2-oxopentanoic acid | C5 H8 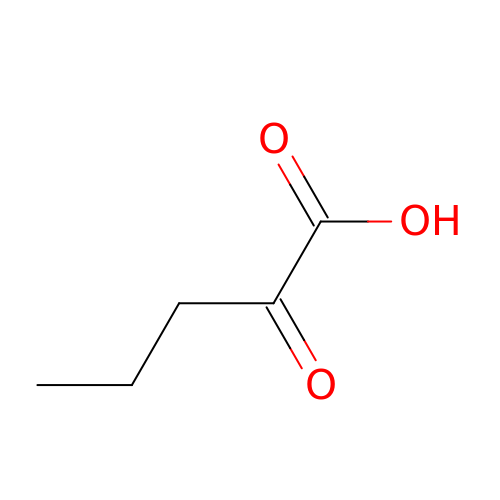O3 | KDVFRMMRZOCFLS-UHFFFAOYSA-N> DWVVAPISVPENGKGPFPQRLNQLKSNKDRDTKIFYSITGPGADSPPEGVFAVEKETGWLLLNKPLDREEIAKYE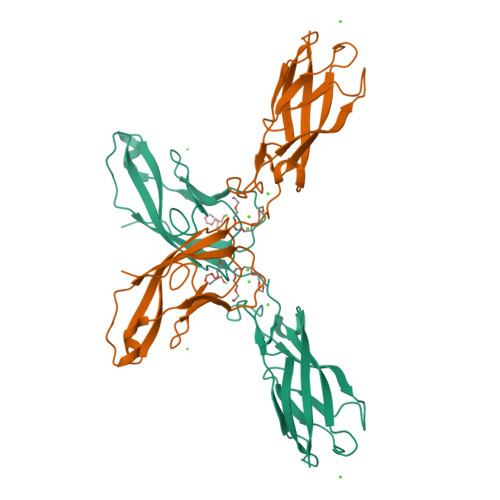LFGHAVSENGASVEDPMNISIIVTDQNDHKPKFTQDTFRGSVLEGVLPGTSVMQVTATDEDDAIYTYNGVVAYSIHSQEPKDPHDLMFTIHRSTGTISVISSGLDREKVPEYTLTIQATDMDGDGSTTTAVAVVEILD~{N}2-methyl-7,8-dihydro-3~{H}-imidazo[4,5-g]quinazoline-2,6-diamine | C10 H12 N6 | 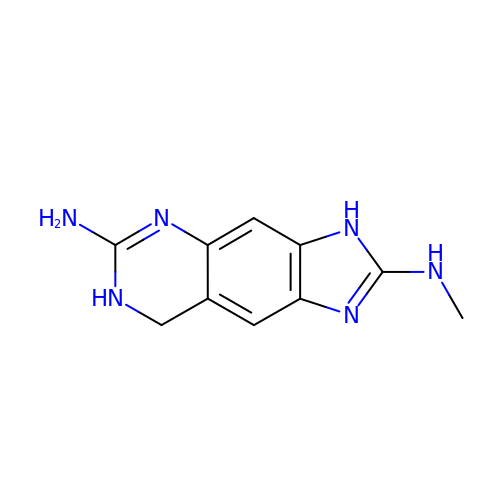WOZSIFRDDMKMGG-UHFFFAOYSA-N>MADNEKLDNQRLKNFKNKGRDLETMRRQRNEVVVELRKNKRDEHLLKRRNVPHEDICEDSDIDGDYRVQNTSLEAIVQNASSDNQGIQLSAVQAARKLLSSDRNPPIDDLIKSGILPILVHCLERDDNPSLQFEAAWALTNIASGTSEQTQAVVQSNAVPLFLRLLHSPHQNVCEQAVWALGNIIGDGPQCRDYVISLGVVKPLLSFISPSIPITFLRNVTWVMVNLCRHKDPPPPMETIQEILPALCVLIHHTDVNILVDTVWALSYLTDAGNEQIQMVIDSGIVPHLVPLLSHQEVKVQTAALRAVGNIVTGTDEQTQVVLNCDALSHFPALLTHPKEKINKEAVWFLSNITAGNQQQVQAVIDANLVPMIIHLLDKGDFGTQKEAAWAISNLTISGRKDQVAYLIQQNVIPPFCNLLTVKDAQVVQVVLDGLSNILKMAEDEAETIGNLIEECGGLEKIEQLQNHENEDIYKLAYEIIDQFFSSDDIDEDPSLVPEAIQGGTFGFNSSANVPTEGFQF[2x];>DKEEVQRKRQKLMP[2x];>DRHRIEEKRKRTYETFKSIMKK[2x]

Nuclear translocation of the p50/p65 heterodimer is essential for NF-κB signaling. Upon activation, p50/p65 is translocated into the nucleus by the adapter importin α3 and the receptor importin β. In the classical pathway, importin α binds to importin β through its N-terminal Importin-β binding (IBB) domain8,9 and to NLS-cargos through its C-terminal 10 stacked Armadillo motifs (Arms) that collectively form an Arm-core. Importin α possesses two NLS binding pockets located along the concave Arm-core surface: an N-terminal ‘major site’ and C-terminal ‘minor site’ between Arms 2–4 and 6–8, respectively.

The best importin α3 crystals diffracted to 2.10 Å for the p50-NLS complex and 2.85 Å with p65/p50-NLS peptides. Interestingly, adding both p65- and p50-NLS peptides to importin α3 and α1 resulted in strong electron density for the p65-NLS peptide at the minor site, with the p50-NLS firmly occupying the major NLS-site. In the importin α3 co-crystal structure with the p65- and p50-NLSs, the eleven residue p65-NLS can be divided into two stretches, with the N-terminal residues 301KRKRT305 adopting an extended conformation and the C-terminal residues 306YETFKS311 folding into an α-helix. The residues 303KRTYE307 occupy the P1′-P5′ positions, including the helical conformation contributing to a salt bridge between p65-NLS Glu307 and importin α3 Lys231 within the Arm 4 coiled region. In contrast, in complex with importin α3, the P2′ position is occupied by Arg304, with Thr305, Tyr306, and Glu307 at the P3′-P5′ positions, respectively. We compared the structures of importin α3 crystallized with different p50- and p65-NLS peptides and found importin α3 adopts a significantly different conformation when the p65-NLS is bound at the minor NLS-box. Similarly, DynDom revealed a shear movement within Arm 7 residues 337–338 only in the importin α3 structure with p65-/p50-NLSs. This shear movement, described as a movement along the plane of an interface, exposes an additional ~93 Å surface area and shifts the C-terminal Arm 10 by ~3.5 Å compared to the apo importin α3 structure. The two chains in the asymmetric unit are nearly identical (RMSD = 1.14 Å), but the dimer is likely a crystallographic artifact due to the high concentration used for crystallization. Both importin α3 molecules in the asymmetric unit are bound to the p50- and p65-NLS peptides, which occupy identical binding sites and have similar structures.> PEYDALFKLLLIGDSGVGKSCLLLRFADDTYTESYISTIGVDFKIRTIELDGKTIKLQIWDTAGQERFRTITSSYYRGAHGII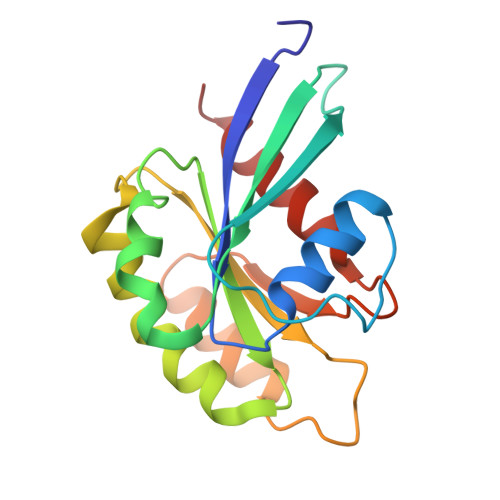VVYDVTDQESFNNVKQWLQEIDRYASENVNKLLVGNKCDLTTKKVVDYTTAKEFADSLGIPFLETSAKNATNVEQSFMTMAAEIKKRM>ASGTSLSAAIHRTQLWFHGRISREESQRLIGQQGLVDGLFLVRESQ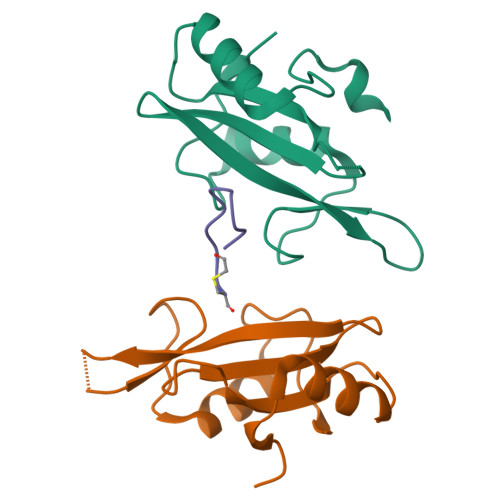RNPQGFVLSLCHLQKVKHYLILPSEEEGRLYFSMDDGQTRFTDLLQLVEFHQLNRGILPCLLRHCCTRVAL[4x];>WFEGYDNTFPC[2x]> GMMVPHLTTALTGPLLTLEKRLLDNMPRIEHWFRSQWQEYGAPFYASVDLRNAGFKLAPVDTNLFPGGFNNLNPDFLPLCIQAAMVAVEKICPDARRLLLIPENHTRNTFYLRNVHALTHILRQAGLEVRIGSIAPEITAPTFLETHDGHSILLEPVRRKANRLELDNFDSCAILLNNDLSGGIPDILQGLEQSLIPPLHAGWATRRKSNHFTAYDRVVEEFAPLIDIDPWLLNPYFDTCGGLDFHARLGEEQLAEKVDSLLAKIRRKYAEYGVKQEPFVIVKADAGTYGMGIMTVKSADDVRDLNRKQRNKMSVVKEGLKVSEVILQEGVYTFEHLKDAVAEPVIYMMDHFVVGGFYRVHTSRGADENLNAPGMHFEPLTFETPCSTPDCAGAPDAAPNRFYAYGVVARL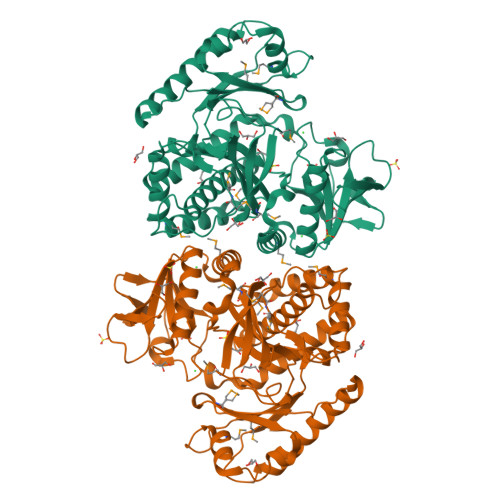ALLAATIELQETDPDLLDERT> MKKAKLGKSDLQVFPIGLGTNAVGGHNLYPNLNEETGKELVREAIRNGVTMLDTAYIYGIGRSEELIGEVLREFNREDVVIATKAAHRKQGNDFVFDNSPDFLK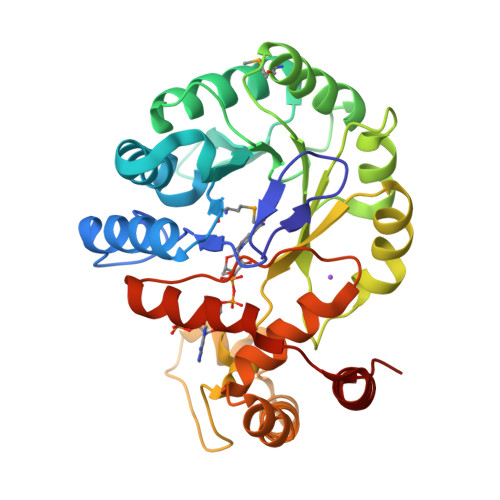KSVDESLKRLNTDYIDLFYIHFPDEHTPKDEAVNALNEMKKAGKIRSIGVSNFSLEQLKEANKDGLVDVLQGEYNLLNREAEKTFFPYTKEHNISFIPYFPLVSGLLAGKYTEDTTFPEGDLRNEQEHFKGERFKENIRKVNKLAPIAEKHNVDIPHIVLAWYLARPEIDILIPGAKRADQLIDNIKTADVTLSQEDISFIDKLFAPG>MLSRKGIIPEEYVLTRLAEDPAEPRYRTRERRARFVSKKGNCNVAHKNIREQGRFLQDVFTTLVDLKWPHTLLIFTMSFLCSWLLFAMVWWLIAFAHGDLAPGEGTNVPCVTSIHSFSSAFLFSIEVQVTIGFGGRMVTEECPLAILILIVQNIVGLMINAIMLGCIFMKTAQAHRRAETLIFSKHAVITLRHGRLCFMLRVGDLRKSMIISATIHMQVVRKTTSPEGEVVPLHQVDIPMENGVGGNGIFLVAPLIIYHVIDSNSPLYDLAPSDLHHHQDLEIIVILEGVVETTGITTQARTSYLADEILWGQRFVPIVAEEDGRYSVDYSKFGNTIKVPTPLCTARQLDEDRSLLDALTLASSRGPLRKRSVAVAKAKPKFSISPDSLS[4x];>MPLAFCGTENHSAAYRVDQGVLNNGCFVDALNVVPHVFLLFITFPILFIGWGSQSSKVHIHHSTWLHFPGHNLRWILTFILLFVLVCEIAEGILSDGVTESRHLHLYMPAGMAFMAAITSVVYYHNIETSNFPKLLIALLIYWTLAFITKTIKFVKFYDHAIGFSQLRFCLTGLLVILYGMLLLVEVNVIRVRRYIFFKTPREVKPPEDLQDLGVRFLQPFVNLLSKGTYWWMNAFIKTAHKKPIDLRAIGKLPIAMRALTNYQRLCVAFDAQARKDTQSPQGARAIWRALCHAFGRRLILSSTFRILADLLGFAGPLCIFGIVDHLGKENHVFQPKTQFLGVYFVSSQEFLGNAYVLAVLLFLALLLQRTFLQASYYVAIETGINLRGAIQTKIYNKIMHLSTSNLSMGEMTAGQICNLVAIDTNQLMWFFFLCPNLWAMPVQIIVGVILLYYILGVSALIGAAVIILLAPVQYFVATKLSQAQRSTLEHSNERLKQTNEMLRGMKLLKLYAWESIFCSRVEVTRRKEMTSLRAFAVYTSISIFMNTAIPIAAVLITFVGHVSFFKESDLSPSVAFASLSLFHILVTPLFLLSSVVRSTVKALVSVQKLSEFLSSAEIREEQCAPREPAPQGQAGKYQAVPLKVVNRKRPAREEVRDLLGPLQRLAPSMDGDADNFCVQIIGGFFTWTPDGIPTLSNITIRIPRGQLTMIVGQVGCGKSSLLLATLGEMQKVSGAVFWNSNLPDSEGEDPSSPERETAAGSDIR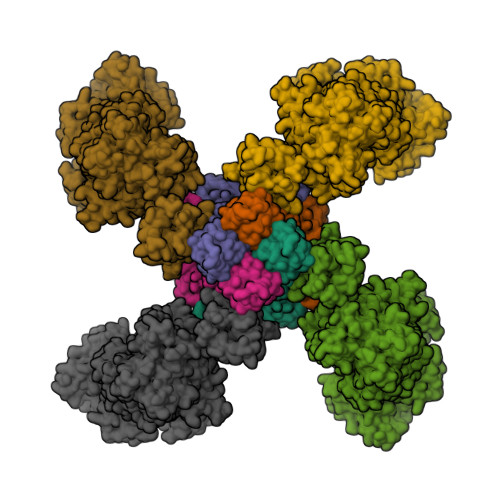SRGPVAYASQKPWLLNATVEENITFESPFNKQRYKMVIEACSLQPDIDILPHGDQTQIGERGINLSGGQRQRISVARALYQQTNVVFLDDPFSALDVHLSDHLMQAGILELLRDDKRTVVLVTHKLQYLPHADWIIAMKDGTIQREGTLKDFQRSECQLFEHWKTLMNRQDQELEKETVMERKASEPSQGLPRAMSSRDGLLLDEEEEEEEAAESEEDDNLSSVLHQRAKIPWRACTKYLSSAGILLLSLLVFSQLLKHMVLVAIDYWLAKWTDSALVLSPAARNCSLSQECDLDQSVYAMVFTLLCSLGIVLCLVTSVTVEWTGLKVAKRLHRSLLNRIILAPMRFFETTPLGSILNRFSSDCNTIDQHIPSTLECLSRSTLLCVSALTVISYVTPVFLVALLPLAVVCYFIQKYFRVASRDLQQLDDTTQLPLLSHFAETVEGLTTIRAFRYEARFQQKLLEYTDSNNIASLFLTAANRWLEVRMEYIGACVVLIAAATSISNSLHRELSAGLVGLGLTYALMVSNYLNWMVRNLADMEIQLGAVKRIHALLKTEAESYEGLLAPSLIPKNWPDQGKIQIQNLSVRYDSSLKPVLKHVNALISPGQKIGICGRTGSGKSSFSLAFFRMVDMFEGRIIIDGIDIAKLPLHTLRSRLSIILQDPVLFSGTIRFNLDPEKKCSDSTLWEALEIAQLKLVVKALPGGLDAIITEGGENFSQGQRQLFCLARAFVRKTSIFIMDEATASIDMATENILQKVVMTAFADRTVVTIAHRVHTILSADLVMVLKRGAILEFDKPETLLSQKDSVFASFVRADK[4x]1-methyl-6-(2-oxidanyl-6-oxidanylidene-cyclohexen-1-yl)carbonyl-3-phenyl-quinazoline-2,4-dione | 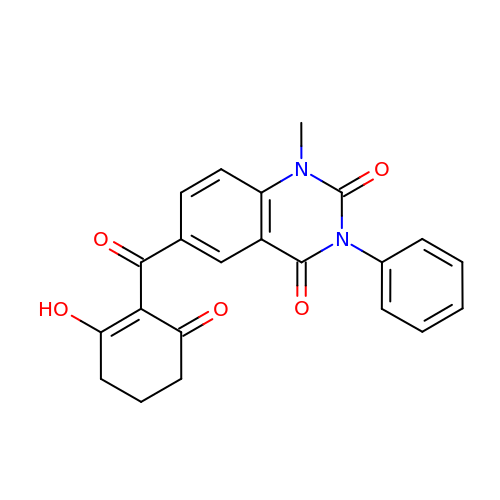C22 H18 N2 O5 | BCNHPWXDPGEOQD-UHFFFAOYSA-N(R)-(4-chloro-2-methoxy-3-{[4-(1H-pyrazol-1-yl)phenyl]methyl}quinolin-6-yl)(1-methyl-1H-imidazol-5-yl)[6-(trifluoromethyl)pyridin-3-yl]methanol 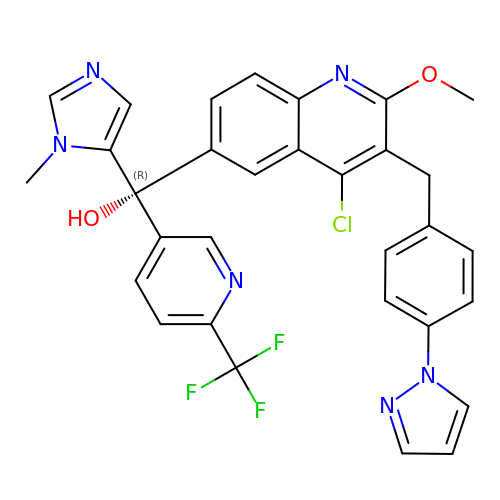| C31 H24 Cl F3 N6 O2 | LZOGZAYEBDXEJA-SSEXGKCCSA-N> MYKDFANFIRTNKKDLLNNWMNEMEKQSDPLINDIAKEPMYEETSIEFVDLIVSNITENGSKFNEKLDDFAEKVVHLGWPIHFVTTGLRVFGLLVYTAMRDEDLFLKREEKPEDD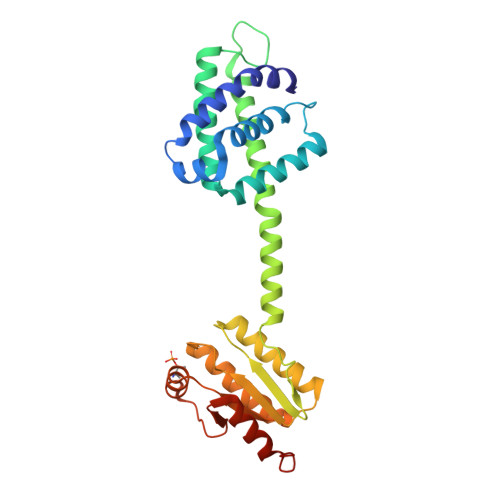AYYRFETWLSSMYNKVVTAYADTWEKTVSIQKSALQELSAPLLPIFEKISVMPLIGTIDTERAKLIIENLLIGVVKNRSEVVLIDITGVPVVDTMVAHHIIQASEAVRLVGCQAMLVGIRPEIAQTIVNLGIELDQIITTNTMKKGMERALALTNREIVEKEG>[2x]DPSKDSKAQVSAAEAGITGTWYNQLGSTFIVT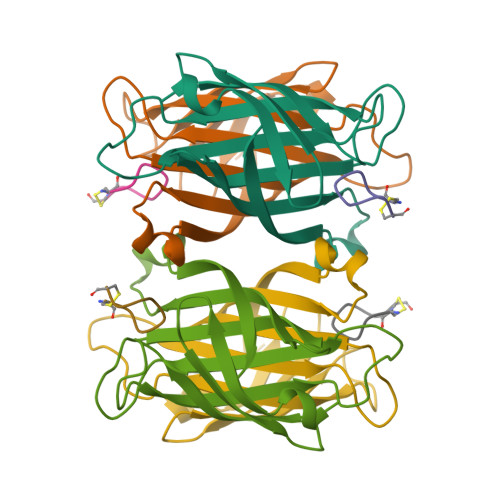AGADGALTGTYESAVGNAESRYVLTGRYDSAPATDGSGTALGWTVAWKNNYRNAHSATTWSGQYVGGAEARINTQWLLTSGTTEANAWKSTLVGHDTFTKVKP;>XCHPQGPPCX[2x]>QQAGTETEEYHLPLTWERDGSSVSASVVIDSNWRWTHSTEDTTNCYDGNEWDSTLCPDADTCTENCAIDGVDQGTWGDTYGITASGSKLTLSFVTEGEYSTDIGSRVFLMADDDNYEIFNLLDKEFSFDVDASNLPCGLNGALYFVSMDEDGGTSKYSTNTAGAKYGTGYCDAQCPHDMKFIAGKANSDGWTPSDNDQNAGTGEMGACCHEMDIWEANSQAQSYTAHVCSVDGYTPCTGTDCGDNGDDRYKGVCDKDGCDYAAYRLGQHDFYGEGGTVDSGSTLTVITQFITGGGGLNEIRRIYQQGGQTIQNAAVNFPGDVDPYDSITEDFCVDIKRYFGDTNDFD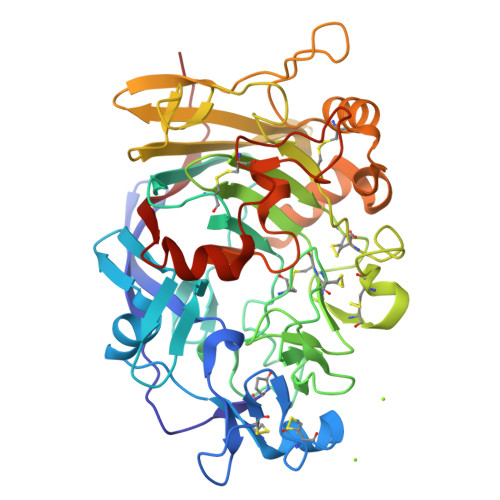AKGGMSGMSNALKKGMVLVMSLWDDHYANMLWLDATYPVDSTEPGALRGPCSTDSGDPADVEANFPGSTVTFSNIKIGPIQSYD[2x]> GSSKKVGTLNRFTQALVIAYVIGYVCVYNKGYQDTDTVLSSVTTKVKGIALTKTSELGERIWDVADYIIPPQEDGSFFVLTNMIITTNQTQSKCAENPTPASTCTSHRDCKRGFNDARGDGVRTGRCVSYSASVKTCEVLSWCPLEKIVDPPNPPLLADAERFTVLIKN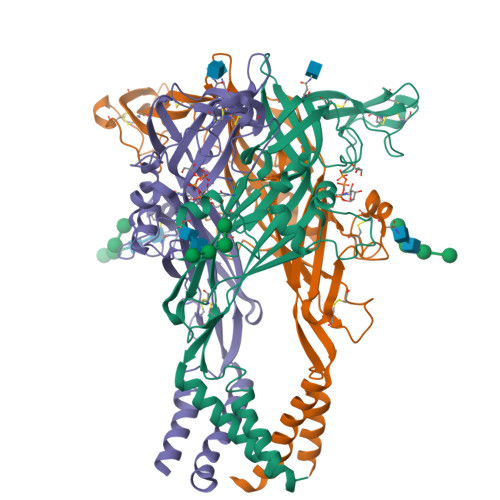NIRYPKFNFNKRNILPNINSSYLTHCVFSRKTDPDCPIFRLGDIVGEAEEDFQIMAVRGGVMGVQIRWDCDLDMPQSWCVPRYTFRRLDNKDPDNNVAPGYNFRFAKYYKNSDGTETRTLIKGYGIRFDVMVFGQAGKFNIIPTLLNIGAGLALLGLVNVICDWIVLTFMK(1S)-1-(3,4-dihydroxybenzyl)-1,2,3,4-tetrahydroisoquinoline-6,7-diol | C16 H17 N O4 | 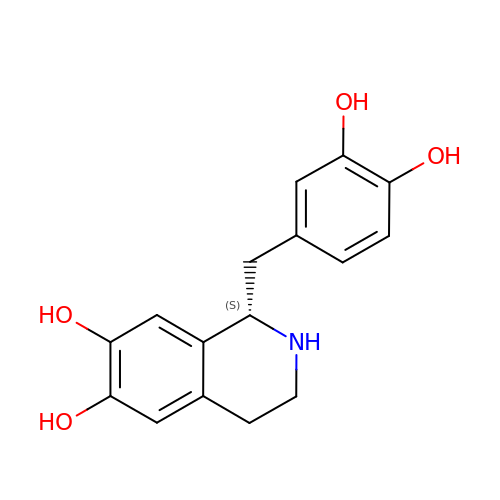ABXZOXDTHTTZJW-LBPRGKRZSA-N> DVSTTGTALRTPAAG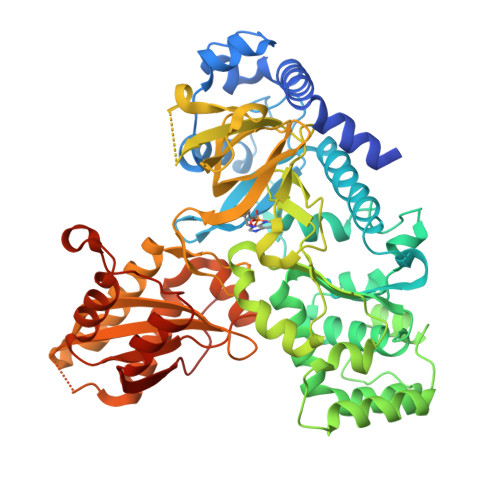AVKEGDVEKLRFIDEMTTNVDAVQERVLGEILGRNAGTEYLTKCGLDGATDRAAFRAKVPVVSYDDLQPYIQRIANGDRSPILSTHPVSEFLTSSGTSAGERKLMPTIMDELDRRQLLYSLLMPVMNLYVPGLDKGKGLYFLFVKSETKTPGGLTARPVLTSYYKSDHFKNRPYDPYHNYTSPTAAILCADAFQSMYAQMVCGLCQRNDVLRLGAVFASGLLRAIRFLQLNWEQLADDIESGELTPRVTDPSVREAVAAILLPDPELAKLIRAECSKGDWAGIITRVWPNTKYLDVIVTGAMAQYIPTLEFYSGGLPMACTMYASSECYFGLNLRPMCDPSEVSYTIMPNMGYFEFLPVDETGAASGDATQLVDLARVEVGREYELVITTYAGLNRYRVGDVLRVTGFHNAAPQFRFVRRKNVLLSIESDKTDEAELQRAVERASALLRPHGASVVEYTSQACTKRIPGHYVIYWELLTKGAGATVVDADTLGRCCLEMEEALNTVYRQSRVADGSIGPLEIRVVRPGTFEELMDYAISRGASINQYKVPRCVTFPPIVELLDSRVVSSHFSPALPHWTPARR>[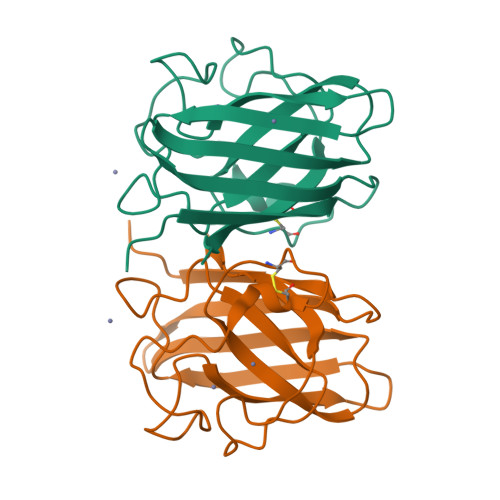4x]QVEGKTQKAVCVIYPTQDYKVTGVITFTKSDDGVKVVADLNGLSPGKHGFHIHECGDCSASDGTSAGGHFNPEEKSHGAPMDMSRHIGDLGNITADENGKAHLEYIDKMIVFEGEHSIIGRSMIVHKNEDDLKTQPTGNAGARVACGVIGIGK> SNAETGAWYMFDEAVEGSTNEFKDYKGNHGNAVLYSANGVVPGLNGNSVSLDGVDDYVALPDGIAGTFYNFTIAFWVRLDTIGEQPIFDFFDSGSNNKYMRLTAESDGKIKFAMTQ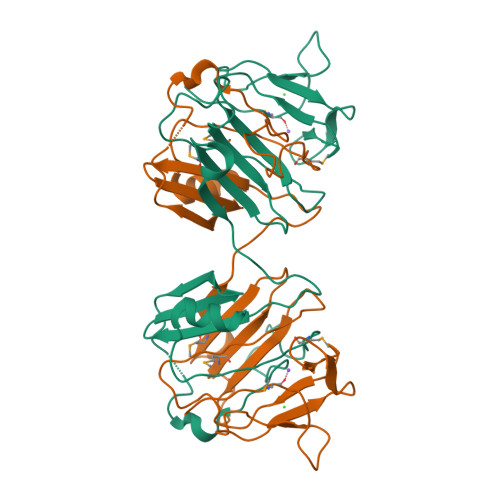SGYYGEKTITSGSALTEGVWKHVAVTLSGDTGTLYINGENVGENNTLSLRPLTFLGETSKGYIGKSHQTDSSEDPYYNSYLHGMIDDFRIFDRALSADEIKTLASVATRVN8-[3-(dimethylamino)phenyl]-~{N}-(4-methylsulfonylpyridin-3-yl)quinoxalin-6-amine 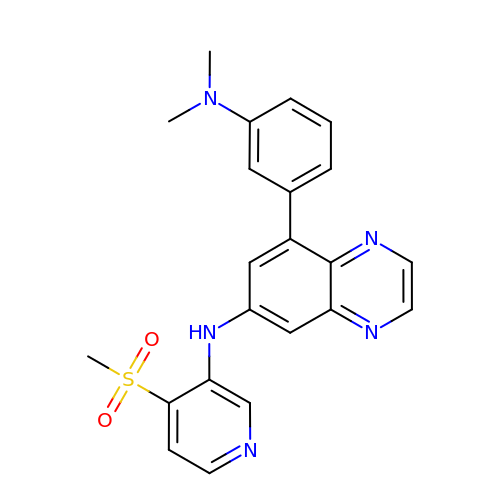| C22 H21 N5 O2 S | MGSNILVOZHNEMV-UHFFFAOYSA-N> LTEE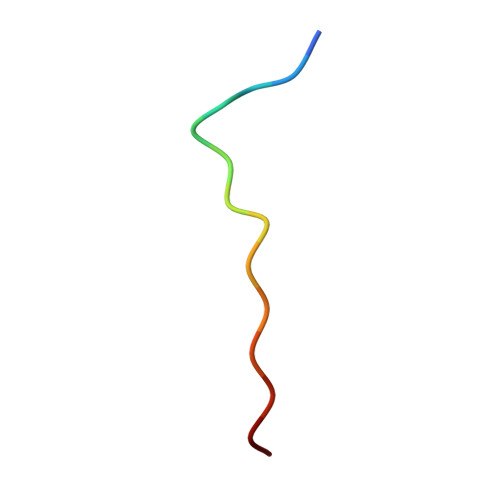LGCDEIIDRE>MTMAKLTESMTNVLEGDSMDQDVESPVAIHQPKLPKQARDDLPRHISRDRTKRKIQRYVRKDGKCNVHHGNVRETYRYLTDIFTTLVDLKWFFNLLIFVMVYTVTWLFFGMIWWLIAYIRGDMDHIEDPSWTPCVTNLNGFVSAFLFSIETETTIGYGYRVITDKCPEGIILLLIQSVLGSIVNAFMVGCMFVKISQPKKRAETLVFSTHAVISMRDGKLCLMFRVGDLRNSHIVEASIRAKLIKSKQTSEGEFIPLNQTDINVGYYTGDDRLFLVSPLIISHEINQQSPFW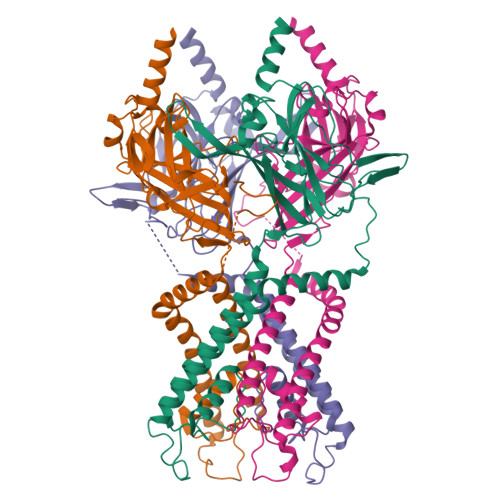EISKAQLPKEELEIVVILEGMVEATGMTCQARSSYITSEILWGYRFTPVLTLEDGFYEVDYNSFHETYETSTPSLSAKELAELANRAESPLSWSVSSKLNQHAELETEEEEKNPEELTERNGDVANLENESKS[4x]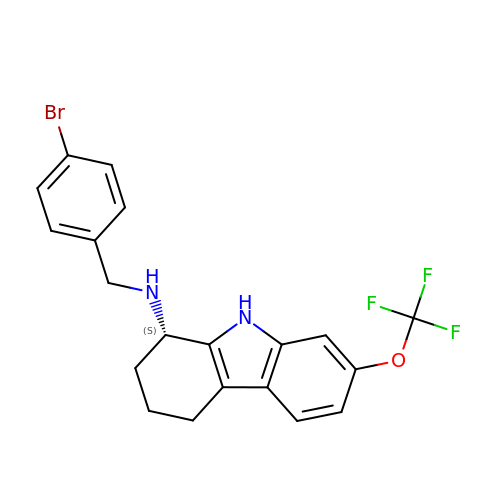(1~{S})-~{N}-[(4-bromophenyl)methyl]-7-(trifluoromethyloxy)-2,3,4,9-tetrahydro-1~{H}-carbazol-1-amine | C20 H18 Br F3 N2 O | YDUCOWUNUQZJIA-KRWDZBQOSA-N N~2~-[(2R,4S,5S)-5-{[N-{[(3,5-DIMETHYL-1H-PYRAZOL-1-YL)METHOXY]CARBONYL}-3-(METHYLSULFONYL)-L-ALANYL]AMINO}-4-HYDROXY-2,7-DIMETHYLOCTANOYL]-N-ISOBUTYL-L-VALINAMIDE 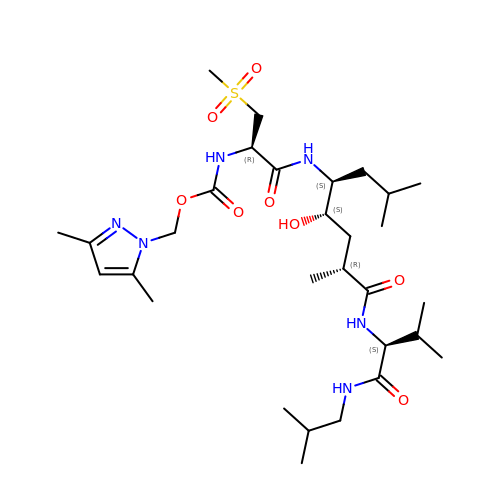| C30 H54 N6 O8 S | OFAZWNGNAATRSH-GWCXRDAXSA-N>[2x]GPAWPEEKNYHQPAILNSSALRQIAEGTSISEMWQNDLQPLLIERYPGSPGSYAARQHIMQRIQRLQADWVLEIDTFLSQTPYGYRSFSNIISTLNPTAKRHLVLACHYDSKYFSHWNNRVFVGATDSAVPCAMMLELARALDKKLLSLKTVSDSKPDLSLQLIFFDGEEAFLHWSPQDSLYGSRHLAAKMASTPHPPGARGTSQLHGMDLLVLLDLIGAPNPTFPNFFPNSA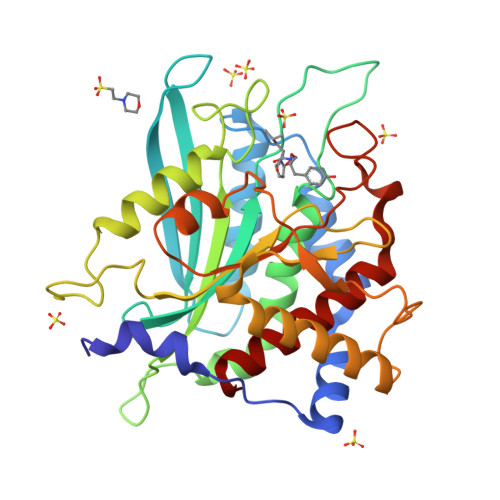RWFERLQAIEHELHELGLLKDHSLEGRYFQNYSYGGVIQDDHIPFLRRGVPVLHLIPSPFPEVWHTMDDNEENLDESTIDNLNKILQVFVLEYLHL> MQDNSRYTHFLTQHYDAKPQGRDDRYCESIMRRRGLTSPCKDINTFIHGNKRSIKAICENKNGNPHRENLRISKSSFQVTTCKLHGGSPWPPC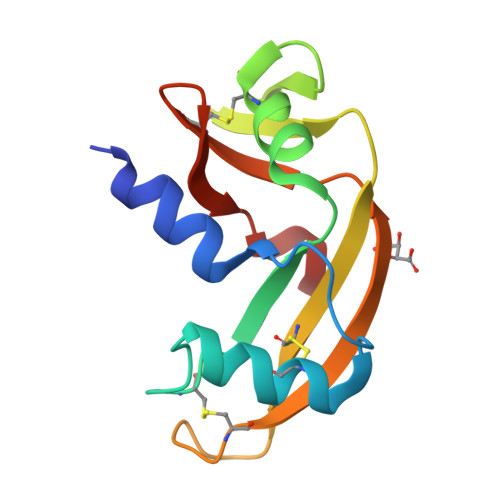QYRATAGFRNIVVACENGLPVHLDQSIFRRP> MAQQIVQSLQDEGTQSLKLDFSMKYVLGYRSDFKNNIFQYTMNDQNRIIYPAGNTIVISNNENKQQFINCIPGTKGITCMTLSPSKRLLAWSEDCDSGIIVVFDLIKLDKLEKAKNQNYQEPSDKDKLDKQAEKDRRDRFEKEKREKIDKLQKEVKRIITTLDCKSRHYVALDFNKINEKRIVALSCAPDWQLIYFQLDKQKTVIINQVPLKVGDNMRYTHCFFHPKEEDFIVAIGTGAIKPYKLGADGQFKQKDPPFVKKESKDQAHSPNYLSYCILQDGYMVIGTDMGEILLFQPSCEFKTILASSPKNEQFAIQCIQPYSKGFLVGGKECTILFYEKDVDLKNPYKLCSKKIQFRDMKAMITSLLLTPNEEKLIVGVDSGQLLQVPFTSDSMQLNEENSKCEPLFMPFHSDKITGLDVCIRKSLVATCSVDKTVRIWNYSDNQLENSKEFEEEAYAVAFHPSGFHIIVAFTEKIRLMNIFENDLISFKELSVKNCREIQFSNGGHFFAITNVSMVQVFQFYTGENPSNLVFRGSGKVRTIFWEEDDQGFYTGSTDGLVIYWRVDDNGPQKTQIAQFNNLIITSITGLYNPDTTTQGLERILFVSGVSSSQENEGEKCVYKLVISCRQDKEGREITDNTLKKIYYVSQPEQKIFTGTNVSQIAISHSKKLFFFATEDRPGAIRITKYPFTNEIMEIQSHFGPITRMRISFKDNYIFTAGEDGALIIYENKEKEYQVKIENESVEAAAEEFLIPRDQYNDQKREIEKLKRQLNEERMKQEQQIKEKMKDRDDKINQLENQQKDSDNRDLNKYQLLEREKNEMIESYEEKKRMMKLQHENN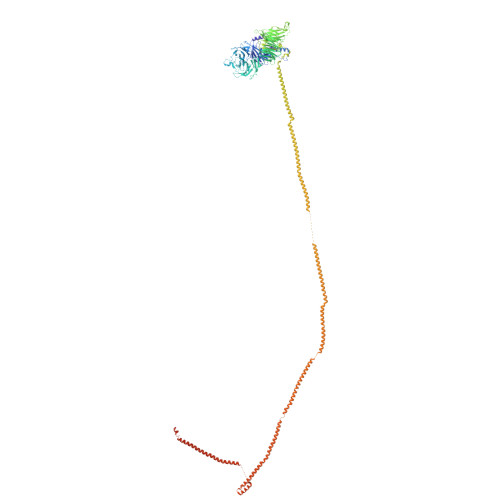KRTIENEYKKKIALEMSRNEELAREKEKEEKRFQSEIQQYQEEHLRQMEEKRRHYEEQLAIEKQLYNDLHLKREELAYKFDQKRNKLEMEAEELIDQLKEENESKMQVLFKNLEKAEIKKMDRRNDYDTEAQKLEEQKSKLKGTMEDITSIQETNKMLQKEKESHAKEIDEREKTIRDKGRRIYELKKKTQELEKFKFVLDYKIKELKRDIGPKEEEIAKMKEQIANMNSEILHFKRTNANLKLIVTDLRLRQEGMKKEIEDQSKVIQQNNQYIKAFEQDMSDCHQHIADYKKLKQKVLNLYNQYVQGDDSKKKRLENNDQQKEIMKERAHLETSVNNLKIKHDKNQSVHKSDTTIIMKHNTFLIFEINHLKREKKKILEDKAKMLMQATQKKKQDGTSRVDIDSLEKEIQKNEDEKRKLKEDIEKLRQYNDQIKNQLRQQIQNQQDDDEDN>GSKKHSVLHLVPVNITSKADSDVTEVMWQPVLRRGRGLEAQGDIVRVWDTGIYLLYSQVLFHDVTFTMGQVVSRE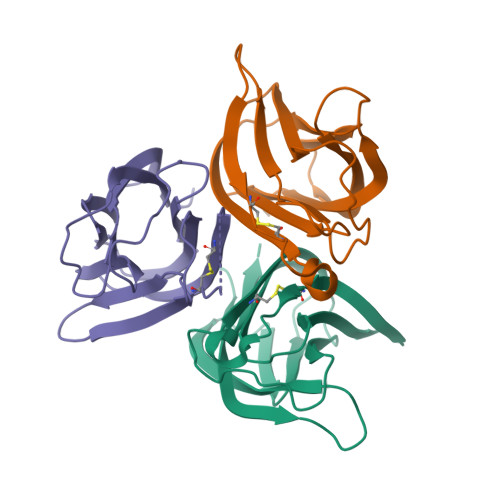GQGRRETLFRCIRSMPSDPDRAYNSCYSAGVFHLHQGDIITVKIPRANAKLSLSPHGTFLGFVKL[3x]>[4x]MGMSMTILPLELIDKCIGSNLWVIMKSEREFAGTLVGFDDYVNIVLKDVTEYDTVTGVTEKHSEMLLNGNGMCMLIPGGKPE;>MGMDSSPNEFLNKVIGKKVLIRLSSGVDYKGILSCLDGYMNLALERTEEYVNGKKTNVYGDAFIRGNNVLYVSALDD[4x];>[4x]GAMGMSSLQKRPGPGNSSQPTERPRKESILDLSRYQDQRIQATFTGGRQIT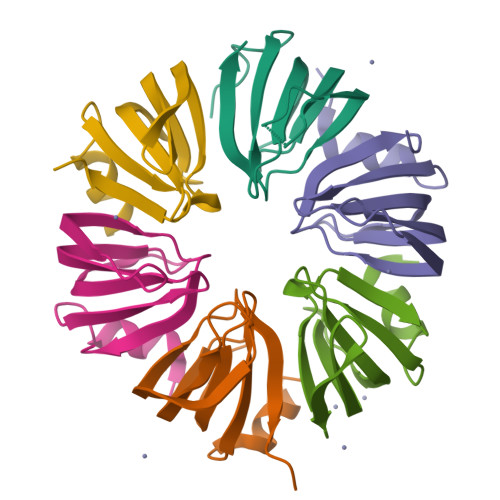GILKGFDQLMNLVLDDVEEQLRNPEDGKLTGAIRKLGLVVVRGTTLVLIAPMDGSEEIPNPFVQAE>GLVPRGSHMSKTRVIYPGTFDPITNGHVDLVTRASRMFDEVVVAIAIGHHKNPLFSLEERVALAQSSLGHLSNVEFVGFDGL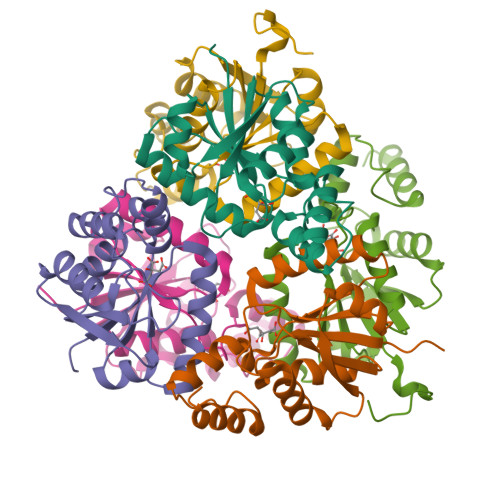LVNFFKEQKATAVLRGLRAVSDFEYEFQLANMNRQLDPHFEAVFLTPSEQYSFISSTLIREIARLKGDVTKFVPQAVVEAFERKHQQGW[6x]> MAAVVKSVALAGRPTTPDRVHEVLGRSMLVDGLDIVLDLTRSGGSYLVDAITGRRYLDMFTFVASSALGMNPPALVDDREFHAELMQAALN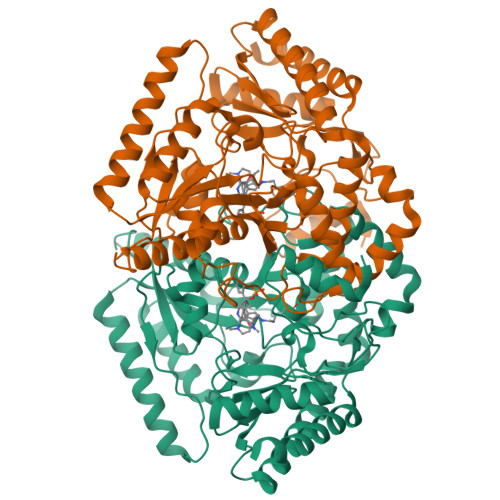KPSNSDVYSVAMARFVETFARVLGDPALPHLFFVEGGALAVENALKAAFDWKSRHNQAHGIDPALGTQVLHLRGAFHGRSGYTLSLTNTKPTITARFPKFDWPRIDAPYMRPGLDEPAMAALEAEALRQARAAFETRPHDIACFVAEPIQGEGGDRHFRPEFFAAMRELCDEFDALLIFDEVQTGCGLTGTAWAYQQLDVAPDIVAFGKKTQVCGVMAGRRVDEVADNVFAVPSRLNSTWGGNLTDMVRARRILEVIEAEGLFERAVQHGKYLRARLDELAADFPAVVLDPRGRGLMCAFSLPTTADRDELIRQLWQRAVIVLPAGADTVRFRPPLTVSTAEIDAAIAAVRSALPVVT> GAGCAGACTAG;> ACACCACTCA;> CTTGT;> TCTGAGTGGAGTCTGC

In this work, we exhaustively probe the ability of all 36 immobile HJ sequences to form DNA crystals in two different designed systems. Three separate self-assembling DNA crystal systems are described in this report: the “4 × 5” and “4 × 6” designs (collectively referred to as the 4 × N systems), and a third construct with a “scrambled” sequence variant of the 4 × 6 lattices. Self-assembly was mediated by three constituent oligonucleotides: (S1) containing four sequence repeats of either 5 or 6 bases; (S2) composed of 21 bases containing complementary regions to both (S1); and (S3) which forms the second junction crossover. The HJ serves as the fundamental component at the core of each unit, and the ultimate assembly of the full lattice is facilitated by the complementary 2-base sticky ends that tail each duplex.

The 4 × 5 system robustly crystallized with 75% of the junctions, and we obtained crystals in all but 9 of 36 sequences. Of the resulting structures, 18 exhibited P32 symmetry with average cell dimensions a = b = 68.85 Å c = 60.09 Å, with only nine retaining the original P3221 symmetry with average cell edges a = b = 68.17 Å c = 60.60 Å. Although the cell parameters between the two symmetries were virtually indistinguishable, the differences between the periodicity of the lattices is dramatic, with vastly different cavity sizes. While the highest resolution achieved for the J1 system was 3.1 Å, in roughly half of the crystals measured the resolutions were 3.05 Å or better, and as high as 2.9 Å (J6) and 2.75 Å (J19), for the P32 and P3221 symmetries, respectively. Pos1 and 2 were readily observable in the electron density maps at either one or both of these conserved sites in a significant number of the structures, with no apparent respect to motif or symmetry. However, in the majority of the crystal structures reported here, the cacodylate anion indeed fits best into the electron density map of our X-ray structures, due to the presence of sodium cacodylate in the crystallization solution.> MISDIRKDAEVRMDKCVEAFKTQISKIRTGRASPSLLDGIVVEYYGTPTPLRQLASVTVEDS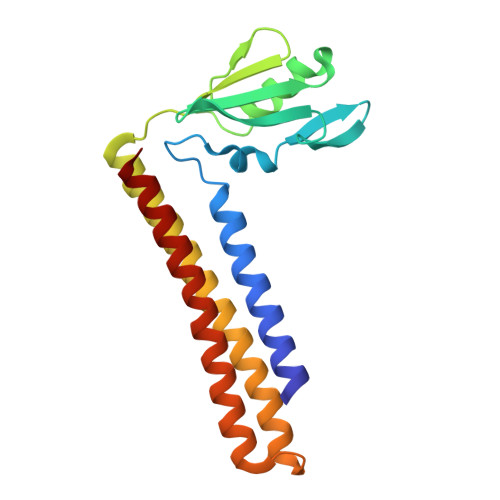RTLKINVFDRSMSPAVEKAIMASDLGLNPNSAGSDIRVPLPPLTEERRKDLTKIVRGEAEQARVAVRNVGRDANDKVKALLKDKEISEDDDRRSQDDVQKLTDAAIKKIEAALADKEAELMQF>[4x]MSFRVSASSSVKPEKDIRIGLLGASGYTGAEIVRLLANHPHFQVTLMTADRKAGQSMESVFPHLRAQKLPTLVSVKDADFSTVDAVFCCLPHGTTQEIIKELPTALKIVDLSADFRLRNIAEYEEWYGQPHKAVELQKEVVYGLTEILREDIKKARLVANPGCYPTTIQLPLVPLLKANLIKHENIIIDAKSGVSGAGRGAKEANLYSEIAEGISSYGVTRHR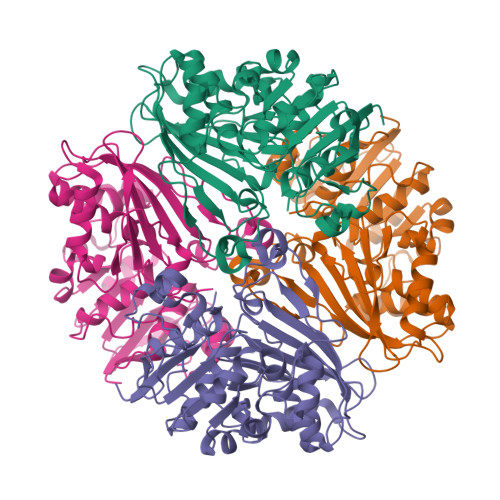HVPEIEQGLSDVAQSKVTVSFTPHLMPMIRGMQSTIYVEMAPGVRTEDLHQQLKTSYEDEEFVKVLDEGVVPRTHNVRGSNYCHMSVFPDRIPGRAIIISVIDNLVKGASGQALQNLNIMLGYPETTGLLHQPLFP> GSHMTDLPRLPFDNPDIMGIAPQMLALQKEGPIARVGTAGEDAWLVTRYDEVRTLLADRRLRLSNPNPQPSAKSAARAFMVALMAGDDHETEPARHAQMRSLLIPRFSTRRLRLMKTRIEHHVDELLDQLAASAPPVDLHRVLSFRLPTMVVCDLLGVPLADRERFGQWARGTFDQS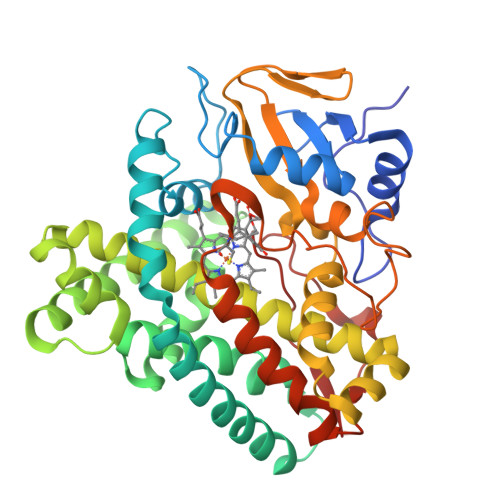DNEHSANTFQQVVDYMLELVARKRVEPGDDILSELIAEKDGALSDADIAHLGNAVLLFGYETTIVRIDLGTLLLLRNPVQRAQLAEDPGLAPAAVEEILRLGVGGKGSNALIPRYAHGDITVGETVIRTGDAVMLAIGAANYDDRAFPDGGLFDLTRVRPRSHLAFGHGARHCIGRTLARIELTAVFERLFRRLPDLRLAVPEESLRWQEHRITGGFDEIPVTF>GSDVVDPDIFNRDPRDHYDLLQRLGGGTYGEVFKARDKVSGDLVALKMVKMEPDDDVSTLQKEILILKTCRHANIVAYHGSYLWLQKLWICMEFCGAGSLQDIYQVTGSLSELQISYVCREVLQGLAYLHSQKKIHRDIKGANILINDAGEVRLADFGISAQIGATLARRLAFIGTPYWMAPEVAAV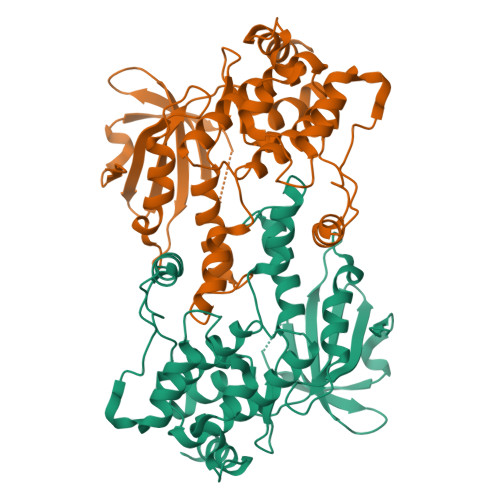ALKGGYNELCDIWSLGITAIELAELQPPLFDVHPLRVLFLMTKSGYQPPRLKEKGKWSAAFHNFIKVTLTKSPKKRPSATKMLSHQLVSQPGLNRGLILDLLDKLKNN[2x]>[4x]MEPEINCSELCDSFPGQELDRRPLHDLCKTTITSSHHSSKTISSLSPVLLGIVWTFLSCGLLLILFFLAFTIHCRKNRIVKMSSPNLNIVTLLGSCLTYSSAYLFGIQDVLVGSSMETLIQTRLSMLCIGTSLVFGPILGKSWRLYKVFTQRVPDKRVIIKDLQLLGLVAALLMADVILLMTWVLTDPIQCLQILSVSMTVTGKDVSCTSTSTHFCASRYSDVWIALIWGCKGLLLLYGAYLAGLTGHVSSPPVNQSLTIMVGVNLLVLAAGLLFVVTRYLHSWPNLVFGLTSGGIFVCTTTINCFIFIPQLKQWKAFEEENQTIRRMAKYFSTPNKSFHTQYGEEENCHPRGEKSSMERLLTEKNAV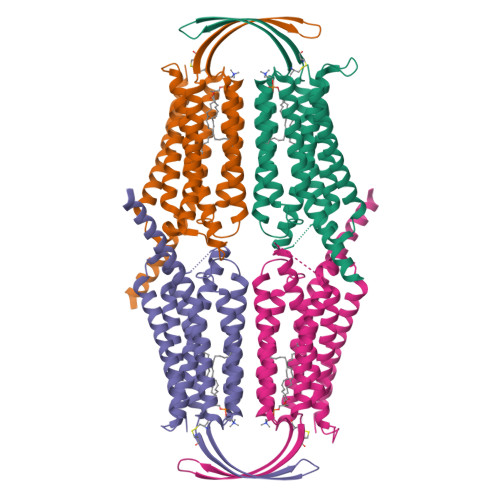IESLQEQVNNAKEKIVRLMSAECTYDLPEGAAPPASSPNKDVQAVASVHTLAAAQGPSGHLSDFQNDPGMAARDSQCTSGPSSYAQSLEGPGKDSSFSPGKEEKISDSKDFSDHLDSGCSQKPWTEQSLGPERGDQVPMNPSQSLLPERGGSDPQRQRHLENSEEPPERRSRVSSVIREKLQEVLQDLGSGSGSGRGRGGSENLYFQGGSGSGGDYKDDDDKDYKDDDDK> MAPVQLDNHQLIPPGGGGGSSGGGGSSSGSASAPAPPPPAAAVAAAAAAAASPG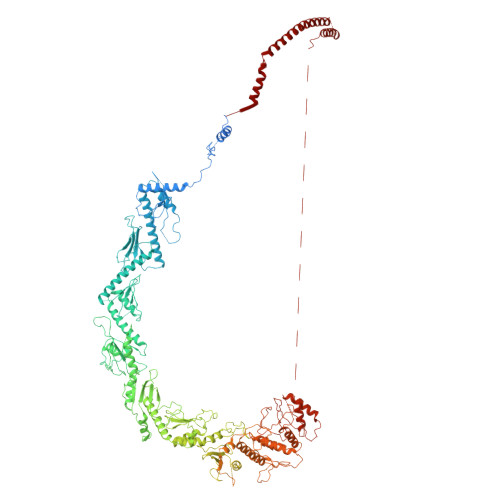YRLSTLIEFLLHRAYSELMVLTDLLPRKSDVERKIEIVQFASRTRQLFVRLLALVKWANDAGKVEKCAMISSFLDQQAILFVDTADRLASLARDALVHARLPSFAIPYAIDVLTTGSYPRLPTCIRDKIIPPDPITKIEKQATLHQLNQILRHRLVTTDLPPQLANLTVANGRVKFRVEGEFEATLTVMGDDPEVPWRLLKLEILVEDKETGDGRALVHSMQIDFIHQLVQSRLFADEKPLQDMYNCLHCFCLSLQLEVLHSQTLMLIRERWGDLVQVERYHAGKSLSLSVWNQQVLGRKTGTASVHKVTIKIDENDVSKPLQIFHDPPLPASDSKLVERAMKIDHLSIEKLLIDSVHARAHQRLQELKAILRSFNANESSSIETALPALIVPILEPCGNSECLHIFVDLHSGMFQLMLYGLDPATLEDMEKSLNDDMKRIIPWIQQLKFWLGQQRCKQSIKHLPTITTETLQLANYSTHPIGSLSKNKLFIKLTRLPQYYIVVEMLEVPNKPTQLSYNYYFMSVSTADREDSPVMALLLQQFKDNIQDLMSYTKTGKQTRTGTKHKLSDDPCPIDSKKAKRSGEMCAFNKVLAHFVAMCDTNMPFVGLRLELSNLEIPHQGVQVEGDGFNHAIRLLKIPPCKGISEETQKALDRSLLDCTFRLQGRNNRTWVAELVFANCPLNGTSTREQGPSRHVYLTYENLLSEPVGGRKVVEMFLNDWSSIARLYECVLEFARSLPEIPAHLNIFSEVRVYNYRKLILCYGTTKGSSISIQWNSIHQKFHIALGTVGPNSGCSNCHNTILHQLQEMFNKTPNVVQLLQVLFDTQAPLNAINKLPTVPMLGLTQRTNTAYQCFSILPQSSTHIRLAFRNMYCIDIYCRSRGVVAIRDGAYSLFDNSKLVEGFYPAPGLKTFLNMFVDSNQDARRRSVNEDDNPPSPIGGDMMDSLISQLQPPQQQPFPKQPGTSGAYPLTSPPTSYHSTVNQSPSMMHTQSPGNLHAASSPSGALRAPSPASFVPTPPPSSHGISIGPGASFASPHGTLDPSSPYTMVSPSGRAGNWPGSPQVSGPSPATRLPGMSPANPSLHSPVPDVSHSPRAGTSSQTMPTNMPPPRKLPQRSWAASIPTILTHSALNILLLPSPTPGLVPGLAGSYLCSPLERFLGSVIMRRHLQRIIQQETLQLINSNEPGVIMFKTDALKCRVALSPKTNQTLQLKVTPENAGQWKPDELQVLEKFFETRVAGPPFKANTLIAFTKLLGAPTHILRDCVHIMKLELFPDQATQLKWNVQFCLTIPPSAPPIAPPGTPAVVLKSKMLFFLQLTQKTSVPPQEPVSIIVPIIYDMASGTTQQADIPRQQNSSVAAPMMVSNILKRFAEMNPPRQGECTIFAAVRDLMANLTLPPGGRPXXXXXXXXXXXXXXXXXXXXXXXXXXXXXXXXXXXXXXXXXXXXXXXXXXXXXXXXXXXXXXXXXXXXXXXXXXXXXXXXXXXXXXXXX>[3x]MAQFDTEYQRLEASYSDSPPGEEDLLVHVAEGSKSPWHHIENLDLFFSRVYNLHQKNGFTCMLIGEIFELMQFLFVVAFTTFLVSCVDYDILFANKMVNHSLHPTEPVKVTLPDAFLPAQVCSARIQENGSLITILVIAGVFWIHRLIKFIYNICCYWEIHSFYLHALRIPMSAL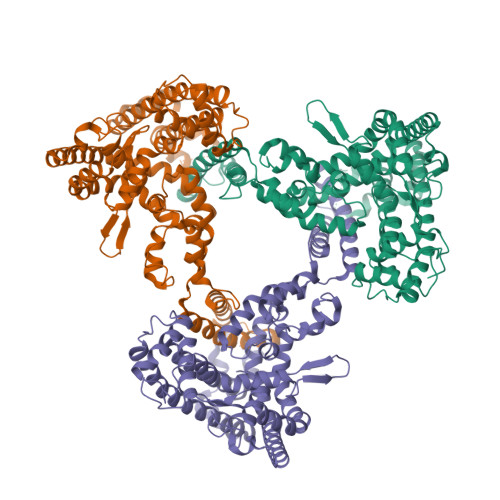PYCTWQEVQARIVQTQKEHQICIHKRELTELDIYHRILRFQNYMVALVNKSLLPLRFRLPGLGEAVFFTRGLKYNFELILFWGPGSLFLNEWSLKAEYKRGGQRLELAQRLSNRILWIGIANFLLCPLILIWQILYAFFSYAEVLKREPGALGARCWSLYGRCYLRHFNELEHELQSRLNRGYKPASKYMNCFLSPLLTLLAKNGAFFAGSILAVLIALTIYDEDVLAVEHVLTTVTLLGVTVTVCRSFIPDQHMVFCPEQLLRVILAHIHYMPDHWQGNAHRSQTRDEFAQLFQYKAVFILEELLSPIVTPLILIFCLRPRALEIIDFFRNFTVEVVGVGDTCSFAQMDVRQHGHPQWLSAGQTEASVYQQAEDGKTELSLMHFAITNPGWQPPRESTAFLGFLKEQVQRDGAAASLAQGGLLPENALFTSIQSLQSESEPLSLIANVVAGSSCRGPPLPRDLQGSRHRAEVASALRSFSPLQPGQAPTGRAHSTMTGSGVDARTASSGSSVWEGQLQSLVLSEYASTEMSLHALYMHQLHKQQAQAEPERHVWHRRESDESGESAPDEGGEGARAPQSIPRSASYPCAAPRPGAPETTALHGGFQRRYGGITDPGTVPRVPSHFSRLPLGGWAEDGQSASRHPEPVPEEGSEDELPPQVHKV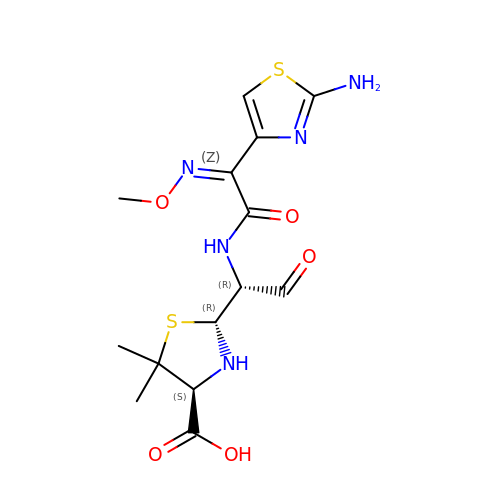2-{1-[2-(2-AMINO-THIAZOL-4-YL)-2-METHOXYIMINO-ACETYLAMINO]-2-OXO-ETHYL}-5,5-DIMETHYL-THIAZOLIDINE-4-CARBOXYLIC ACID | C14 H19 N5 O5 S2 | YVNKGXXVZIQNIV-RKMXGKDGSA-N>[2x]GSHMADKELKFLVVDDFSTMRRIVRNLLKELGFNNVEE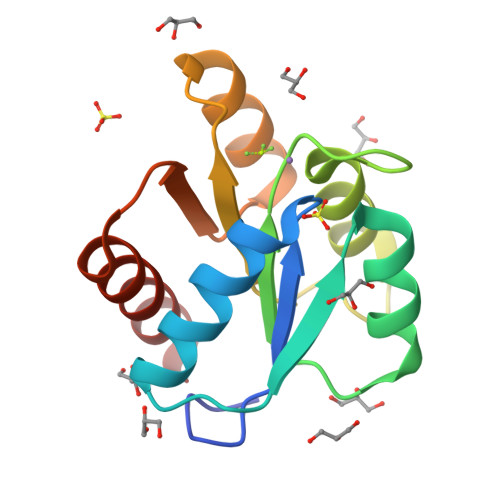AEDGVDALNKLQAGGYGFVISDWDMPNMDGLELLKTIRADGAMSALPVLMVTAQAKKENIIAAAQAGASGYVVKPFTAATLEEKLNKIFEKLGM>GSWNEPYFDLTMPRNITSLVGKSAYLGCRVKHLGNKTVAWIRHRDLHILTVGTYTYTTDQRFQTSYHRDIDEWTLQIKWAQQRDAGVYECQISTQPVRSYSVNLNIVHHHHHH[2x];>[2x]SRAFQPEFVESISNVSVAVGRDAT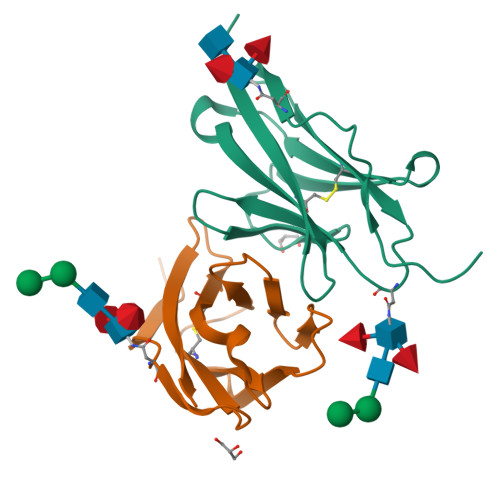FTCHVRHLGGYRVGWLKADTKAIQAIHENVITHNPRVTVSHLDQNTWNLHIKAVSEEDRGGYMCQLNTDPMKSQIGFLDVVIPHHHHHH>TTIVSVRRNGHVVIAGDGQATLGNTVMKGNVKKVRRLYNDKVIAGFAGGTADAFTLFELFERKLEMHQGHLVKAAVELAKDWRTDRMLRKLEAL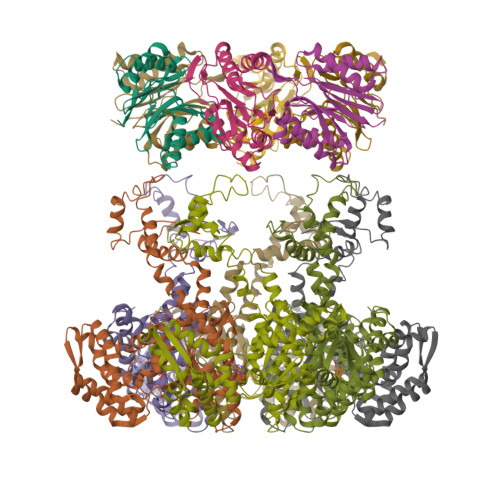LAVADETASLIITGNGDVVQPENDLIAIGSGGPYAQAAARALLENTELSAREIAEKALDIAGDICIYTNHFHTIEELSYKA[8x];>HHHHHHHSEMTPREIVSELDKHIIGQDNAKRSVAIALRNRWRRMQLNEELRHEVTPKNILMIGPTGVGKTEIARRLAKLANAPFIKVEATKFTEVGYVGKEVDSIIRDLTDAAVKMVRVQAIEKNRYRAEELAEERILDVLIPPAKNNWGQTEQQQEPSAARQAFRKKLREGQLDDKEIEIDLAAAPMGVEIMAPPGMEEMTSQLQSMFQNLGGQKQKARKLKIKDAMKLLIEEEAAKLVNPEELKQDAIDAVEQHGIVFIDEIDKICKRGESSGPDVSREGVQRDLLPLVEGCTVSTKHGMVKTDHILFIASGAFQIAKPSDLIPELQGRLPIRVELQALTTSDFERILTEPNASITVQYKALMATEGVNIEFTDSGIKRIAEAAWQVNESTENIGARRLHTVLERLMEEISYDASDLSGQNITIDADYVSKHLDALVADEDLSRFIL[4x]> MDVVSLDKPFMYFEEIDNELDYEPES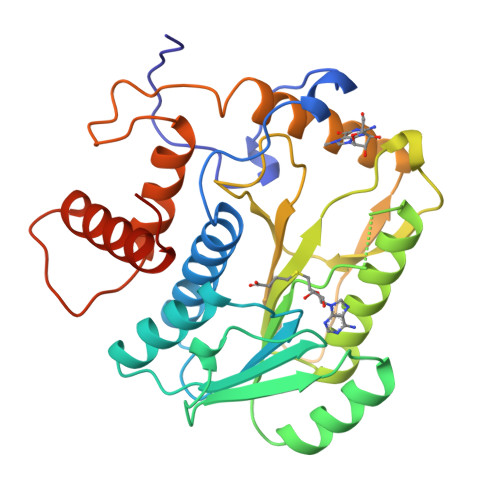ANEVAKKLPYQGQLKLLLGELFFLSKLQRHGILDGATVVYIGSAPGTHIRYLRDHFYNLGVIIKWMLIDGRHHDPILNGLRDVTLVTRFVDEEYLRSIKKQLHPSKIILISDVRSKRGGNEPSTADLLSNYALQNVMISILNPVASSLKWRCPFPAQWIKDFYIPHGNKMLQPFAPSYSAEMRLLSIYTGENMRLTRVTKSDAVNYEKKMYYLNKIVRNKVVVNFDYPNQEYDYFHMYFMLRTVYCNKTFPTTKAKVLFLQQSIFRFLNIPTTSTEKVSHE> MREMLQVERPKLILDDGKRTDGRKPDELRSIKIELGVLKNADGSAIFEMGNTKAIAAVYGPKEMHPRHLSLPDRAVLRVRYHMTPFST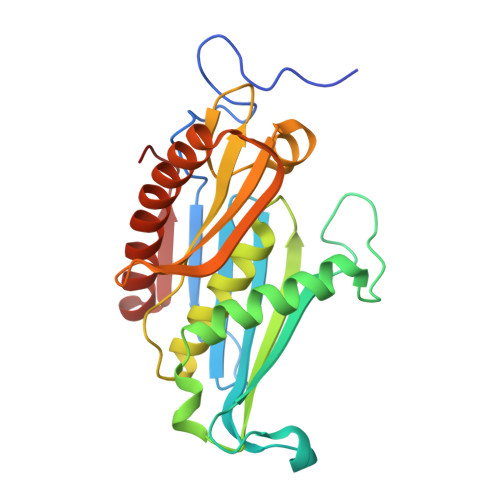DERKNPAPSRREIELSKVIREALESAVLVELFPRTAIDVFTEILQADAGSRLVSLMAASLALADAGIPMRDLIAGVAVGKADGVIILDLNETEDMWGEADMPIAMMPSLNQVTLFQLNGSMTPDEFRQAFDLAVKGINIIYNLEREALKSKYVEFKEEGV> MKDQLSDEQKETILKALNDAIE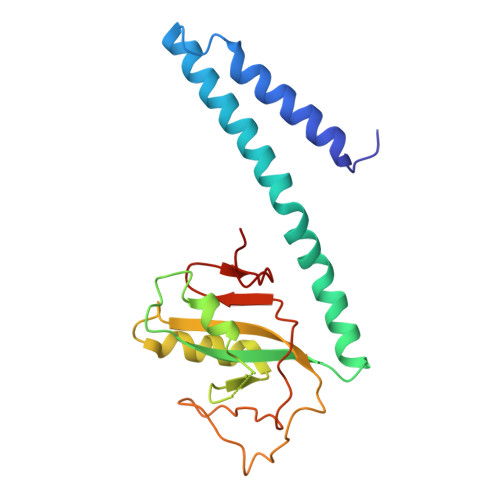KGPWDKSNFLRVIGKKLIAIRDRFLKRIGAASQAQLQAESHLANQIALQSGQQEIYVSLYSSDGSNLQSWEKIVGSLPRQMISRPIYADEEDIKAILKTKENKQNEAYVAIYISQSDILHLSADKAPVDKLGKPLLTLKDKSISLENISRFVHVSGVYRYSNGRLIKNA> MAPEINLPGPMSLIDNTKGQLVVNPEALKILSAITQPVVVVAIVGLYRTGASYLMNKLAGKKNGFSLGSTVKSHTKGIWMWCVPHPKKPEHTLVLLDTEGLGDIEKGDNENDSWIFALAILLSSTFVYNSMGTINQQAMDQLHYVTELTDRIKANSSPGNNSVDDSADFVSFFPAFVWTLRDFTLELEVDGEPITADDYLELSLKLRKGTDKKSKSFNDPRLCIRKFFPKRKCFVFDWPAPKKYLAHLEQLKEEELNPDFIEQVAEFCSYILSHSNVKTLSGGIPVNGPRLESLVLTYVNAISSGDLPCRENAVLALAQIENSAAVEKAIAHYEQQMGQKVQLPTETLQELLDLHRDSEREAIEVFMKNSFKDVDQMFQRKLGAQLEARRDDFCKQNSKASSDCCMALLQDIFGPLEEDVKQGTFSKPGGYRLFTQKLQEL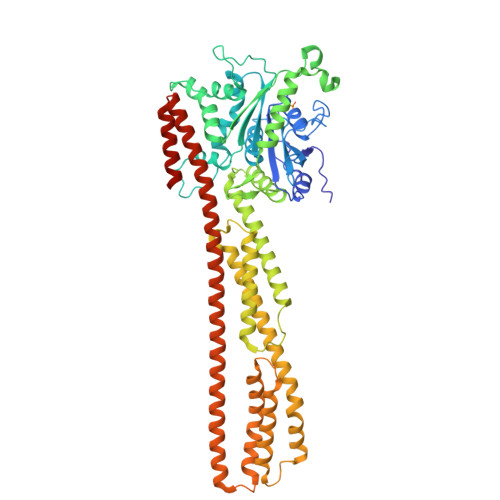KNKYYQVPRKGIQAKEVLKKYLESKEDVADALLQTDQSLSEKEKAIEVERIKAESAEAAKKMLEEIQKKNEEMMEQKEKSYQEHVKQLTEKMERDRAQLMAEQEKTLALKLQEQERLLKEGFENESKRLQKDIWDIQMRSKSLEPICNIL> MEIVYKPLDIRNEEQFASIKKLIDADLSEPYSIYVYRYFLNQWP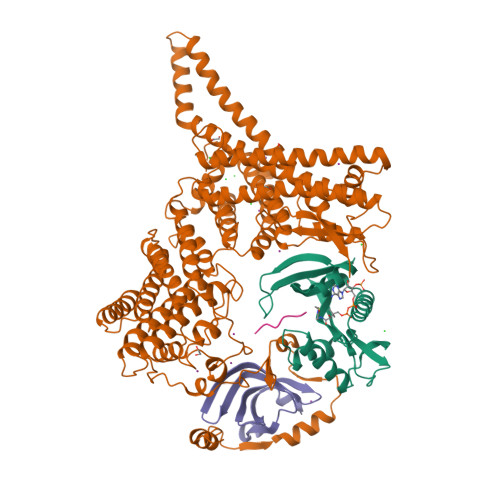ELTYIAVDNKSGTPNIPIGCIVCKMDPHRNVRLRGYIGMLAVESTYRGHGIAKKLVEIAIDKMQREHCDEIMLETEVENSAALNLYEGMGFIRMKRMFRYYLNEGDAFKLILPLT;> GPMEVDSILGSLSITDDFDQLVDVTSLFDELCSKLKPEAIVKDPRFDLFEGTHSLEVNNSKLDSSLIELTAEEIEFDVNVAYDPPLASVAAIADRLLRCVISWLNDYQTLPTTVLSCRYTESLLSSLVKGTTAGSSWCTGNILYDKVLGSCILGVCYLTKFVQKLLSAGIVFEEEDLNFNNMGFNTFDNLPGQDVVINSLTESLQILEAYSDDSLHLTMLKHILKIIICLVHLEDHLTDYSTKTSHLDELIENANSVNGIFPQLQLSPPKGAFSTYIQKHRSNQFPPRKITKLPTDYSGFITLANDVKTILLVDKAESALETYQFAKFFNKLEQRHVIARILFPLFFIRDDRTVLGKFSYTQFYLLHVKEFSAQTPSEFESSIGNELIQESSNMLLEWYQNCSQNTCRYRQGFNRQLILWDSLQAQFESVNSQVYCSWTYFMKLSSMIEFSLKGFDLDIYKPFEAYSMFWYVYYLSHHLETFLKDSQNDIESNINAIHSMNKKLKKLKAGEKKDQLRLKYRFAMDNEMEQLQATKQFLNYLLKEINITKSLCLIEVFQFAILKSFGLIDNKNSTPSKFSNERLIHNLRFKPFNSIGVPELPEYEVFQQTLKDFVIEEKGAAFDIKLERATNFIETEVRNVVSSIDEIMQGIKGGDNNGVLVTGTRLVQELSLEYYCKLKHTSKALSVNSKVIVNTLKKNIKNKDSHEYKVELVHTTEGWNYFPIQTLRIKQDRYK;> MDILKLSDFIGNTLIVSLTEDRILVGSLVAVDAQMNLLLDHVEERMGSSSRMMGLVSVPRRSVKTIMIDKPVLQELT;> MLRFVGSRRR>[2x]SGIVVSPILIPENQRQPFPRDVGKVVDSDRPEGSKFRLTGKGVDQDPKGTFRINENTGS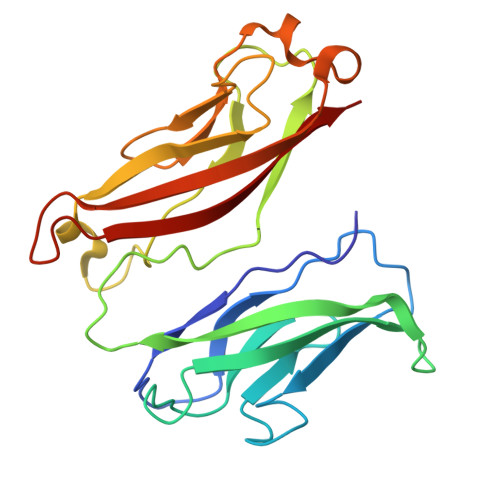VSVTRTLDRETIATYQLYVETTDASGKTLEGPVPLEVIVIDQNDNRPIFREGPYIGHVMEGSPTGTTVMRMTAFDADDPATDNALLRYNIRQQTPDKPSPNMFYIDPEKGDIVTVVSPALLDRETLENPKYELIIEAQDMAGLDVGLTGTATATIVIDD> 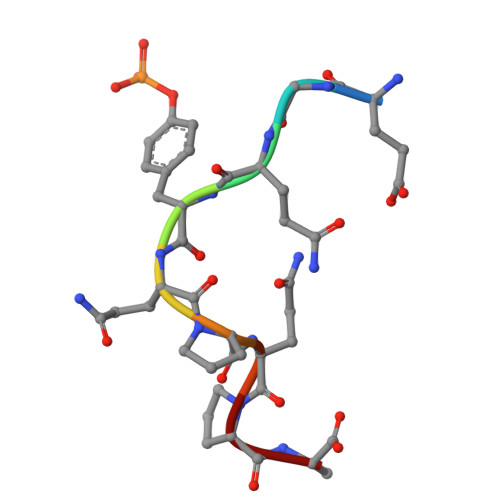EGQYQPQPA> PISPIETVPVKLKPGMDGPKVKQWPLTEEKIKALVEICTEMEKEGKISKIGPENPYNTPVFAIKKKDSTKWRKLVDFRELNKRTQDFWEVQLGIPHPAGLKKKKSVTVLDVGDAYFSVPLDEDFRKYTAFTIPSINNETPGIRYQYNVLPQGWKGSPAIFQSSMTKILEPFKKQNPDIVIYQYMDDLYVGSDLEIGQHRTKIEELRQHLLRWGLTTPDKKHQKEPPFLWMGYELHPDKWTVQPIVLPEKDSWTVNDIQKLVGKLNWASQIYPGIKVRQLCKLLRGTKALTEVIPLTEEAELELAENREILKEPVHGVYYDPSKDLIAEIQKQGQGQWTYQIYQEPFKNLKTGKYARMRGAHTNDVKQLTEAVQKITTESIVIWGKTPKFKLPIQKETWETWWTEYWQATWIPEWEFVNTPPLVKLWYQLEKEPIVGAETFYVDGAANRETKLGKAGYVTNKGRQKVVPLTNTTNQKTQLQAIYLALQDSGLEVNIVTDSQYALGIIQAQPDKSESELVNQIIEQLIKKEKVYLAWVPAHKGIGGNEQVDKLVSAGIRKIL;> PISPIETVPVKLKPGMDGPKVKQWPLTEEKIKALVE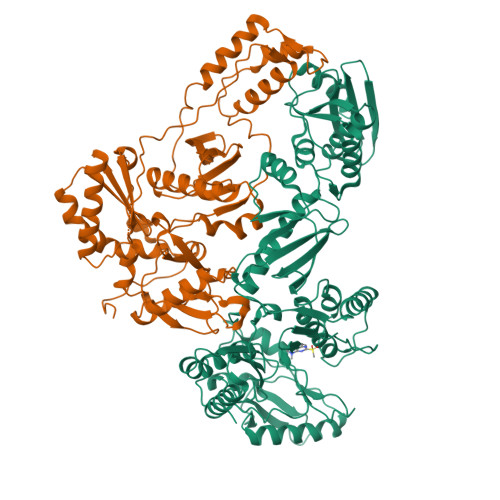ICTEMEKEGKISKIGPENPYNTPVFAIKKKDSTKWRKLVDFRELNKRTQDFWEVQLGIPHPAGLKKKKSVTVLDVGDAYFSVPLDEDFRKYTAFTIPSINNETPGIRYQYNVLPQGWKGSPAIFQSSMTKILEPFKKQNPDIVIYQYMDDLYVGSDLEIGQHRTKIEELRQHLLRWGLTTPDKKHQKEPPFLWMGYELHPDKWTVQPIVLPEKDSWTVNDIQKLVGKLNWASQIYPGIKVRQLCKLLRGTKALTEVIPLTEEAELELAENREILKEPVHGVYYDPSKDLIAEIQKQGQGQWTYQIYQEPFKNLKTGKYARMRGAHTNDVKQLTEAVQKITTESIVIWGKTPKFKLPIQKETWETWWTEYWQATWIPEWEFVNTPPLVKLWY>MATTGTPTADRGDAAATDDPAARFQVQKHSWDGLRSIIHGSRKYSGLIVNKAPHDFQFVQKTDESGPHSHRLYYLGMPYGSRENSLLYSEIPKKVRKEALLLLSWKQMLDHFQATPHHGVYSREEELLRERKRLGVFGITSYDFHSESGLFLFQASNSLFHCRDGGKNGFMVSPMKPLEIKTQCSGPRMDPKICPADPAFFSFINNSDLWVANIETGEERRLTFCHQGLSNVLDDPKSAGVATFVIQEEFDRFTGYWWCPTASWEGSEGLKTLRILYEEVDESEVEVIHVPSPALEERKTDSYRYPRTGSKNPKIALKLAEFQTDSQGKIVSTQEKELVQPFSSLFPKVEYIARAGWTRDGKYAWAMFLDRPQQWLQLVLLPPALFIPSTENEEQRLASARAVPRNVQPYVVYEEVTNVWINVHDIFYPFPQSEGEDELCFLRANECKTGFCHLYKVTAVLKSQGYDWSEPFSPGEDEFKCPIKEEIALTSGEWEVLARHGSKIWVNEETKLVYFQGTKDTPLEHHLYVVSYEAAGEIVRLTTPGFSHSCSMSQNFDMFVSHYSSVSTPPCVHVYKLSGPDDDPLHKQPRFWASMMEAASCPPDYVPPEIFHFHTRSDVRLYGMIYKPHALQPGKKHPTVLFVYGGPQVQLVNNSFKGIKYLRLNTLASLGYAVVVIDGRGSCQRGLRFEGALKNQMGQVEIEDQVEGLQFVAEKYGFIDLSRVAIHGWSYGGFLSLMGLIHKPQVFKVAIAGAPVTVWMAYDTGYTERY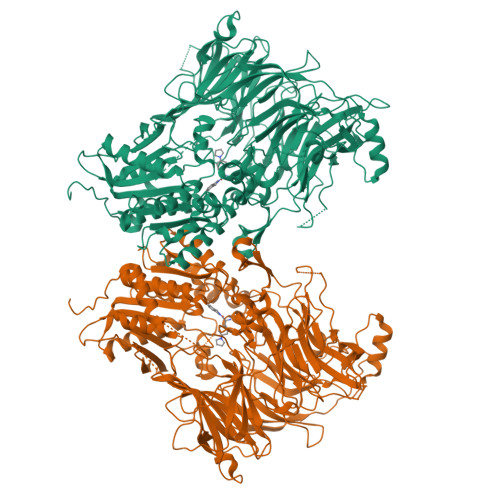MDVPENNQHGYEAGSVALHVEKLPNEPNRLLILHGFLDENVHFFHTNFLVSQLIRAGKPYQLQIYPNERHSIRCPESGEHYEVTLLHFLQEYLHHHHHH[4x]>GELVRTDSPNFLCSVLPTHW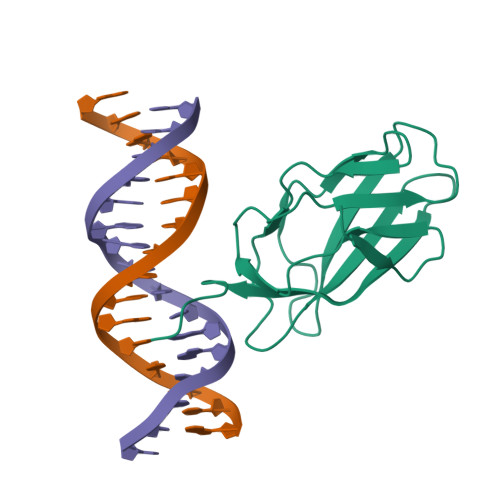RCNKTLPIAFKVVALGDVPDGTLVTVMAGNDENYSAELRNATAAMKNQVARFNDLRFVGRSGRGKSFTLTITVFTNPPQVATYHRAIKITVDGPREPRRHRQK[2x]> MKRIPRKTKGKSSGKGNDSTERADDGSSQLRDKQNNKAGPATTEPGTSNREQYKARPGIASVQRATESAEMPMKNNDEGTPDKKGNTKGDLVNEHSEAKDEADEATKKQAKDTDKSKAQVTYSDTGINNANELSRSGNVDNEGGSNQKPMSTRIAEATSAIVSKHPARVGLPPTASSGHGYQCHVCSAVLFSPLDLDAHVASHGLHGNMTLTSSDIQRHITEFISSWQNHPIV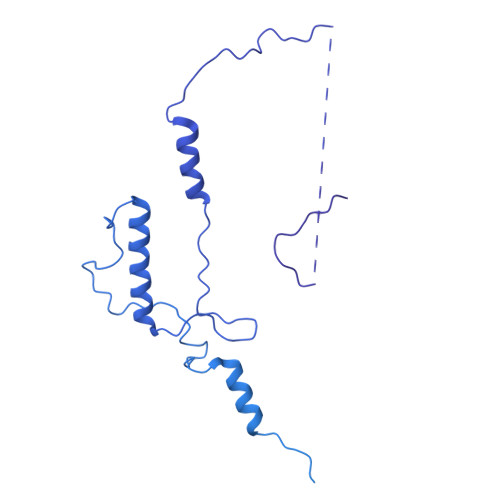QVSADVENKKTAQLLHADTPRLVTWDAGLCTSFKIVPIVPAQVPQDVLAYTFFTSSYAIQSPFPEAAVSRIVVHTRWASNVDFDRDSSVIMAPPTENNIHLFKQLLNTETLSVRGANPLMFRANVLHMLLEFVLDNLYLNRHTGFSQDHTPFTEGANLRSLPGPDAEKWYSIMYPTRMGTPNVSKICNFVASCVRNRVGRFDRAQMMNGAMSEWVDVFETSDALTVSIRGRWMARLARMNINPTEIEWALTECAQGYVTVTSPYAPSVNRLMPYRISNAERQISQIIRIMNIGNNATVIQPVLQDISVLLQRISPLQIDPTIISNTMSTVSESTTQTLSPASSILGKLRPSNSDFSSFRVALAGWLYNGVVTTVIDDSSYPKDGGSVTSLENLWDFFILALALPLTTDPCAPVKAFMTLANMMVGFETIPMDNQIYTQSRRASAFSTPHTWPRCFMNIQLISPIDAPILRQWAEIIHRYWPNPSQIRYGAPNVFGSANLFTPPEVLLLPIDHQPANVTTPTLDFTNELTNWRARVCELMKNLVDNQRYQPGWTQSLVSSMRGTLDKLKLIKSMTPMYLQQLAPVELAVIAPMLPFPPFQVPYVRLDRDRVPTMVGVTRQSRDTITQPALSLSTTNTTVGVPLALDARAITVALLSGKYPPDLVTNVWYADAIYPMYADTEVFSNLQRDMITCEAVQTLVTLVAQISETQYPVDRYLDWIPSLRASAATAATFAEWVNTSMKTAFDLSDMLLEPLLSGDPRMTQLAIQYQQYNGRTFNIIPEMPGSVIADCVQLTAEVFNHEYNLFGIARGDIIIGRVQSTHLWSPLAPPPDLVFDRDTPGVHIFGRDCRISFGMNGAAPMIRDETGLMVPFEGNWIFPLALWQMNTRYFNQQFDAWIKTGELRIRIEMGAYPYMLHYYDPRQYANAWNLTSAWLEEITPTSIPSVPFMVPISSDHDISSAPAVQYIISTEYNDRSLFCTNSSSPQTIAGPDKHIPVERYNILTNPDAPPTQIQLPEVVDLYNVVTRYAYETPPITAVVMGVP> SMQGPRTRARLGANEVLLVVGGFGSQQSPIDVVEKYDPKTQEWSFLPSITRKRRYVASVSLHDRIYVIGGYDGRSRLSSVECLDYTADEDGVWYSVAPMNVRRGLAGATTLGDMIYVSGGFDGSRRHTSMERYDPNIDQWSMLGDMQTAREGAGLV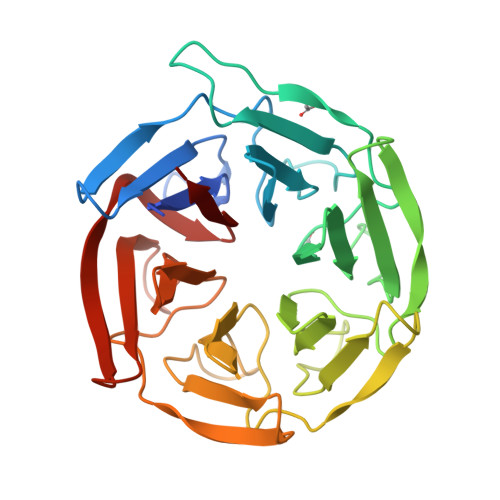VASGVIYCLGGYDGLNILNSVEKYDPHTGHWTNVTPMATKRSGAGVALLNDHIYVVGGFDGTAHLSSVEAYNIRTDSWTTVTSMTTPRCYVGATVLRGRLYAIAGYDGNSLLSSIECYDPIIDSWEVVTSMGTQRCDAGVCVLRE>TPAFNKPKVELHVHLDGAIKPETILYFGKKRGIALPADTVEELRNIIGMDKPLSLPGFLAKFDYYMPVIAGCREAIKRIAYEFVEMKAKEGVVYVEVRYSPHLLANSKVDPMPWNQTEGDVTPDDVVDLVNQGLQEGEQAFGIKVRSILCCMRHQPSWSLEVLELCKKYNQKTVVAMDLAGDETIEGSSLFPGHVEAYEGAVKNGIHRTVHAGEVGSPEVVREAVDILKTERVGHGYHTIEDEALYNRLLKENMHFEVCPWSSYLTGAWDPK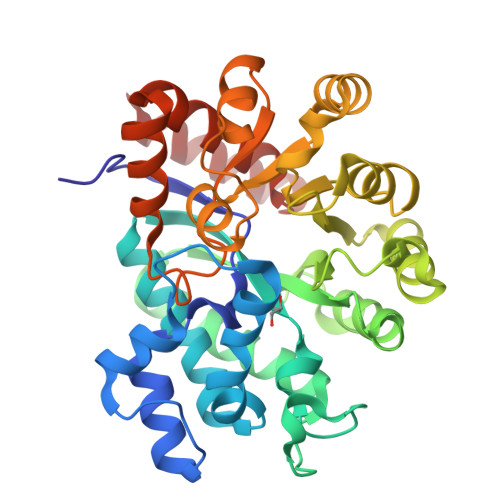TTHAVVRFKNDKANYSLNTDDPLIFKSTLDTDYQMTKKDMGFTEEEFKRLNINAAKSSFLPEEEKKELLERLYREYQ[2x]> MKEITFKINGQEMIVPEGTTILEAARMNNIDIPTLCYLKDINEIGACRMCLVEIAGARALQAACVYPVANGIEVLTNSPKVREARRVNLELILSNHNRECTTCIRSENCELQTLATDLGVSDIPFEGEKSGKLIDDLSTSVVRDESKCILCKRCVSVCRDVQSVAVLGTVGRGFTSQVQPVFNKSLADVGCINCGQCIINCPVGALKEKSDIQRVWDAIADPSKTVIVQTAPAVRAALGEEFGYPMGTSVTGKMAAALRRLGFDKVFDTDFGADVCIMEEGTELIGRVTNGGVLPMITSCSPGWIKFIETYYPEAIPHLSSCKSPQNITGALLKNHYAQTNNIDPKDMVVVSIMPCTAKKYEVQREELCTDGNADVDISITTRELARMIKEARILFNKLPDEDFDDYYGESTGAAVIFGATGGVMEAAVRTVADVLNKKDIQEIDYQIVRGVDGIKKASVEVTPDLTVNLVVAHGGANIREV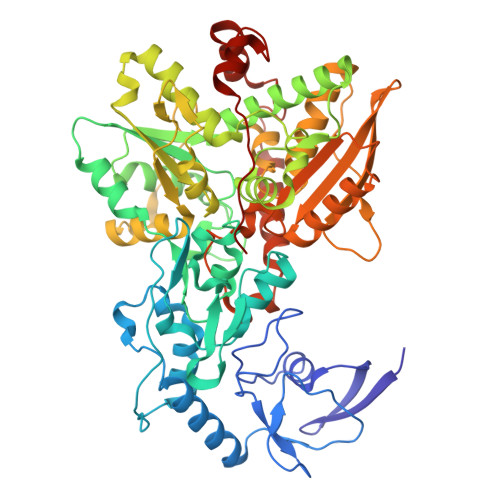MEQLKAGELADTHFIELMACPGGCVNGGGQPIVSAKDKMDIDIRTERAKALYDEDANVLTYRKSHQNPSVIRLYEEYLEEPNSPKAHHILHTKYSAKPKLV> MKEFYLTVEQIGDSIFERYIDSNGRERTREVEYKPSLFAHCPESQATKYFDIYGKPCTRKLFANMRDASQWIKRMEDIGLEALGMDDFKLAYLSDTYNYEIKYDHTKIRVANFDIEVTSPDGFPEPSQAKHPIDAITHYDSIDDRFYVFDLLNSPYGNVEEWSIEIAAKLQEQGGDEVPSEIIDKIIYMPFDNEKELLMEYLNFWQQKTPVILTGWNVESFAIPYVYNRIKNIFGESTAKRLSPHRKTRVKVIENMYGSREIITLFGISVLDYIDLYKKFSFTNQPSYSLDYISEFELNVGKLKYDGPISKLRESNHQRYISYNIIAVYRVLQIDAKRQFINLSLDMGYYAKIQIQSVFSPIKTWDAIIFNSLKEQNKVIPQGRSHPVQPYPGAFVKEPIPNRYKYVMSFDLTSLYPSIIRQVNISPETIAGTFKVAPLHDYINAVAERPSDVYSCSPNGMM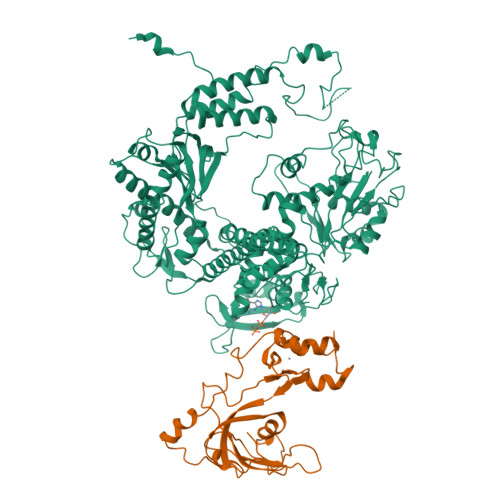YYKDRDGVVPTEITKVFNQRKEHKGYMLAAQRNGEIIKEALHNPNLSVDEPLDVDYRFDFSDEIKEKIKKLSAKSLNEMLFRAQRTEVAGMTAQINRKLLINSLYGALGNVWFRYYDLRNATAITTFGQMALQWIERKVNEYLNEVCGTEGEAFVLYGDTDSIYVSADKIIDKVGESKFRDTNHWVDFLDKFARERMEPAIDRGFREMCEYMNNKQHLMFMDREAIAGPPLGSKGIGGFWTGKKRYALNVWDMEGTRYAEPKLKIMGLETQKSSTPKAVQKALKECIRRMLQEGEESLQEYFKEFEKEFRQLNYISIASVSSANNIAKYDVGGFPGPKCPFHIRGILTYNRAIKGNIDAPQVVEGEKVYVLPLREGNPFGDKCIAWPSGTEITDLIKDDVLHWMDYTVLLEKTFIKPLEGFTSAAKLDYEKKASLFDMFDF;> MKGFSSEDKGEWKLKLDASGNGQAVIRFLPAKTDDALPFAILVNHGFKKNGKWYIETCSSTHGDYDSCPVCQYISKNDLYNTNKTEYSQLKRKTSYWANILVVKDPQAPDNEGKVFKYRFGKKIWDKINAMIAVDTEMGETPVDVTCPWEGANFVLKVKQVSGFSNYDESKFLNQSAIPNIDDESFQKELFEQMVDLSEMTSKDKFKSFEELNTKFNQVLGTAALGGAAAAAAS> MRGSHHHHHHGSLSSSPSEILQELGKGSTHPQPGVSPPAAPAAPGPKDGPGETDAFGNSEGKELVASGENKIKQGLLPSLEDLLFYTIAEGQEKIPVHKFITALKSTGLRTSDPRLKECMDMLRLTLQTTSDGVMLDKDLFKKCVQSNIVLLTQAFRRKFVIPDFMSFTSHIDELYESAKKQSGGKVADYIPQLAKFSPDLWGVSVCTADGQRHSTGDTKVPFCLQSCVKPLKYAIAVNDLGTEYVHRYVGKEPSGLRFNKLFLNEDDKPHNPMVNAGAIVVTSLIKQGVNNAEKFDYVMQFLNKMAGNEYVGFSNATFQSERESGDRNFAIGYYLKEKKCFPEGTDMVGILDFYFQLCSIEVTCESASVMAATLANGGFCPITGERVLSPEAVRNTLSLMHSCGMYDFSGQFAFHVGLPAKSGVAGGILLVVPNVMGMMCWSPPLDKMGNSVKGIHFCHD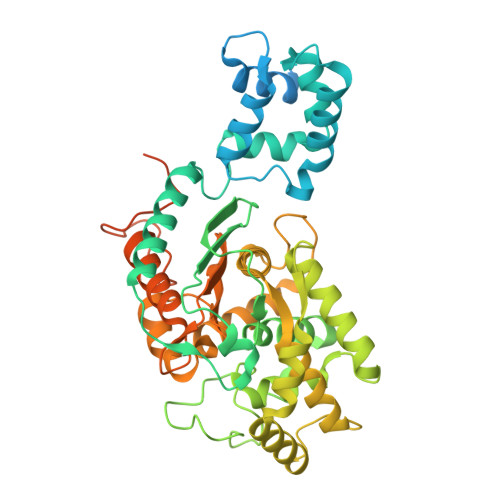LVSLCNFHNYDNLRHFAKKLDPRREGGDQRHSFGPLDYESLQQELALKETVWKKVSPESNEDISTTVVYRMESLGEKS>VPMGKFAMYPDWQPDADFIRLAALWGVALREPVTTEELASFIAYWQAEGKVFHHVQWQQKLARSLQIGRAS[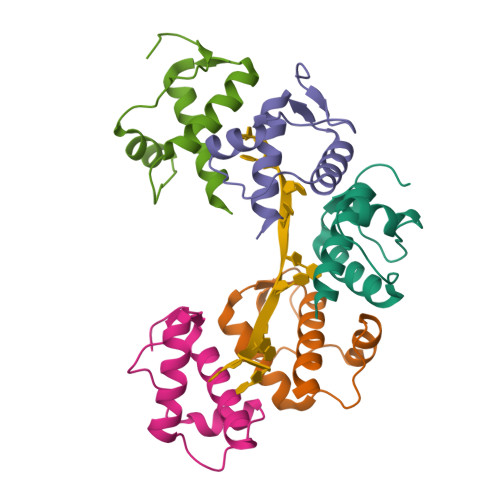5x]> HALQLKPGQP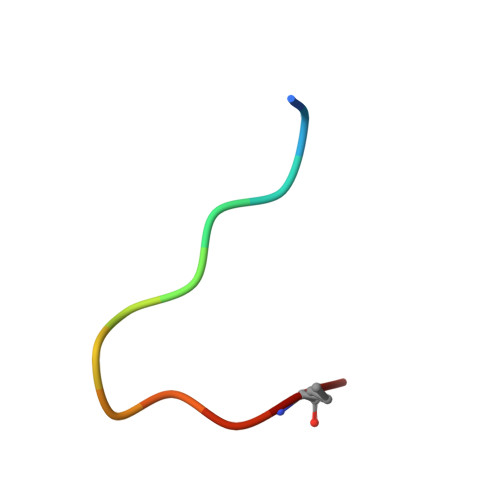LY>MSKPSIVILGAGYGGIVAALGLQKRLNYNEADITLVNKNDYHYITTELHQPAAGTMHHDQARVGIKELIDEKKIKFVKDTVVAIDREQQKVTLQNGELHYDYLVVGLGSEPETFGIEGLREHAFSINSINSVRIIRQHIEYQFAKFAAEPERTDYLTIVVGGAGFTGIEFVGELADRMPELCAEYDVDPKLVRIINVEAAPTVLPGFDPALVNYAMDVLGGKGVEFKIGTPIKRCTPEGVVIEVDGEEEEIKAATVVWTGGVRGNSIVEKSGFETMRGRIKVDPYLRAPGHENIFIVGDCAL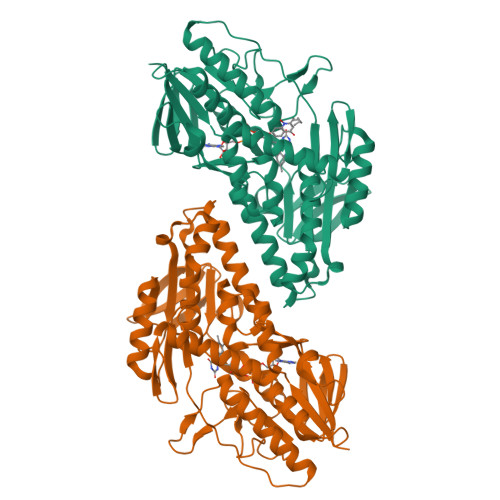IINEENNRPYPPTAQIAIQHGENVAANLAALIRGGSMTPFKPHIRGTVASLGRNDAIGIVGGRKVYGHAASWLKKLIDMRYLYLIGGLSLVLKKGRFHHHHHH[4x]The bacterial proteins of the Dsb family catalyze the formation of disulfide bridges between cysteine residues that stabilize protein structures and ensure their proper functioning. The oxidative part of this network consists of two monomeric DsbAs (DsbA1 and DsbA2) related to EcDsbL, which cooperate with one DsbB. The solved structures of both CjDsbAs, especially the length and amino acid sequences of their L2 and L3 loops that are essential elements of the monomeric thiol oxidoreductases, were different from that of EcDsbA but similar, though not identical, to that of EcDsbL, which affected their functioning.

CjDsbA1 crystallized in the C2 and P212121 space group containing two monomers in the ASU for the monoclinic form and one molecule per ASU for the orthorhombic form, while CjDsbA2 crystallized in P3221 with a single chain in the ASU. In the orthorhombic CjDsbA1, the electron density map allowed for the building of the residue range 5–193. The superposition of monoclinic and orthorhombic forms of CjDsbA1 showed relatively small differences between them, which was confirmed by an RMSD value of 0.45 Å. The active site of CjDsbA1 was observed in the reduced form, while the CjDsbA2 formed a clear disulfide bond. This was due to differences in protein purification procedures. CjDsbA1 was purified under reducing conditions. It should be noted that the CjDsbA1 redox potential was the highest among the characterized DsbAs so far described; EcDsbL has a redox potential of −95 mV and N. meningitidis lipoprotein NmDsbA2 has a redox potential of −79 mV. We found that only CjDsbA1 restored E. coli ΔdsbA resistance to cadmium. In contrast, CjDsbA1 complemented a lack of EcDsbA in an EcDsbB-dependent manner. CjDsbA1 in E. coli was partially oxidized, probably due to sulfonic acid, and generated oligomeric forms (resolved by CjDsbB) that are active in disulfide generation.

> MANNSFITLNPSLPNSENSVIEAFSYKCIHCYNHHKFGTLEKLREAFPNLHFKLYPVSLMNGEFSKEMNELFAFAQYKDEQNGKDASYSDSLSHKLADVYFVSYFLNKQRNFSNLDEFYDIGLKAMNVNKNEVLNFLNTPKAKEILSEFQRANDIAKTYGTPAFVVNGKYQINPSAINSMQDLEDLVKKLSNMKLEHHHHHH> GERPYMQPFHLIPPSLSVQATEQPLASNEAWDYPEPLAPGQSPAASSEEGSSEEKGDEREPHGDEGKRGRKDKKKSKTQRIASAVNGLGFRLYKQVLGGAGPADNIFFSPLSIASALGVVTAGANGSTRAELDTALGFKEFLHGKKKAKSMKYFARLNGALYKRSAGFELMGKNVVFSKKGLWLYRQFTRTVAHLFKSNVRSVDFGDSKNAVELMNAYIEKVTSKKFPDVISDVDTDTSLVIVNVIYFKGSWGNKFEPDLTKNVRFWVNSSYSMMVPTMHQRAKLSYTQ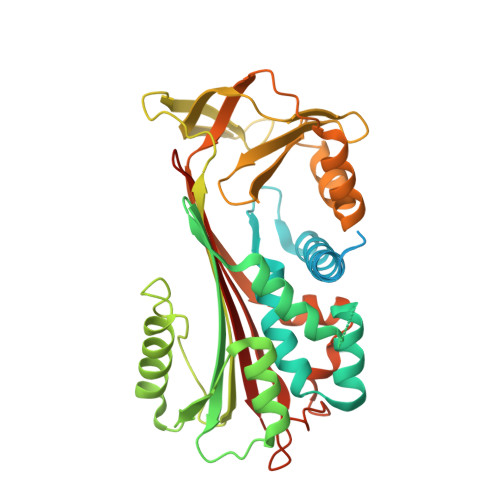DRKLRSTVVKLPYEGGASMLVIVPHRTEDLPKVEESVSQEQLEEWLSLLGPSNHYVQLSLPKFKISVSYDLKAYLSAMGMSSMFSYGADLSRITGMQKLHVDKITHKSVLHVNEEGTEAKAETVVGIMAAPR2-(4-phenoxyphenoxy)ethyl thiocyanate | C15 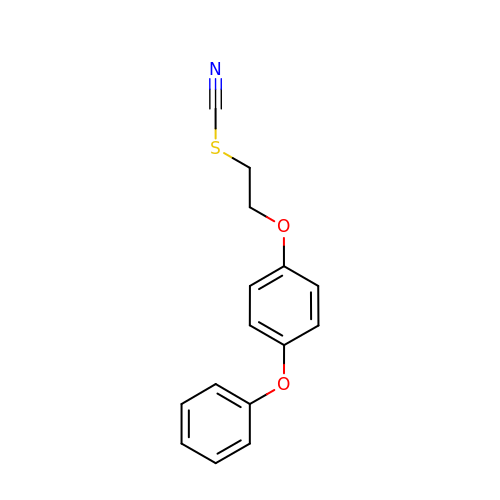H13 N O2 S | YQZHGQYIMXWEHI-UHFFFAOYSA-N> TLVHVASVEK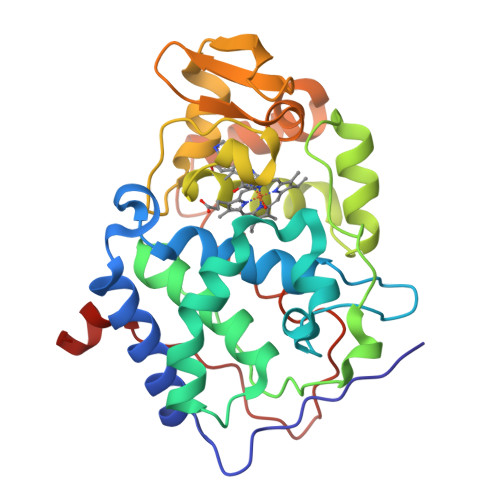GRSYEDFQKVYNAIALKLREDDEYDNYIGYGPVLVRLAWHISGTWDKHDNTGGSYGGTYRFKKEFNDPSNAGLQNGFKFLEPIHKEFPWISSGDLFSLGGVTAVQEMQGPKIPWRCGRVDTPEDTTPDNGRLPDADKDAGYVRTFFQRLNMNDREVVALMGAHALGKTHLKNSGYEGGGANNVFTNEFYLNLLNEDWKLEKNDANNEQWDSKSGYMMLPTDYSLIQDPKYLSIVKEYANDQDKFFKDFSKAFEKLLENGITFPKDAPSPFIFKTLEEQGL> MFHFTVGSLKNLNSWYAKGTMRGGVPRIYYAWMRPGSFTRRRFEKMRNPFVDLETGTSLYFRDTRDSAEAVAHAADSKGLKGMDNAIDLYNEYRIVPDLYPEGFQWKHKLNTEYNQWRSNTWLTPDLIPQEHRGRFLCNFQLNIVAYDMRVVKFSPKDHRQWIYCVLYVGSGKGIAGWGRAVAPSTQEAKKEAIREAFSNIIAVDLEQEGPMYPVRVNADGVRVLLYPAKRIVANFRVADILCAFGFQHAGCRINL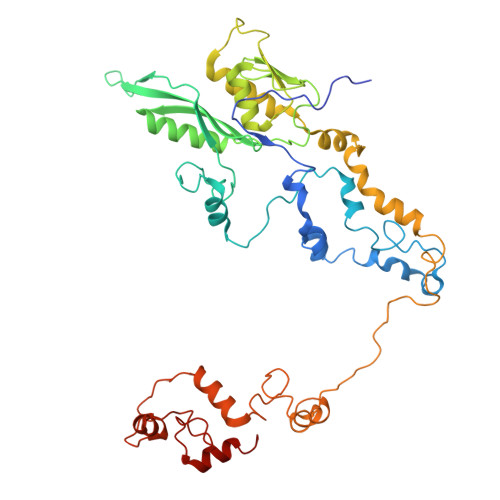KATNNPKSPTHTVEGVFEAVKALRSVSEIAASRGKVPHSLIYNIYPYLEEIRRRKGMMAMHPPGKDGLLMPDRVVDNRLPDHLKKGYYDDVYWKDFFAGSREHLNEPKMGLRGDEMRQRLESAQSRPISSSTGSGRRTLEDVLKRLGKTTKDLGSIPIVNPRLDIKLPTHIKRNYSLH>[2x]SMQDPTIFEERHLKYISQLGKGNFGSVELCRYDPLGDNTGALVAVKQLQHSGPDQQRDFQREIQILKALHSDFIVKYRGVSYGPGRQSLRLVMEYLPSGCLRDFLQRHRARLDASRLLLYSSQICKGMEYLGSRRCVHRALAARNILVESEAHVKIADFGLAKLLPLDKDYYVVREP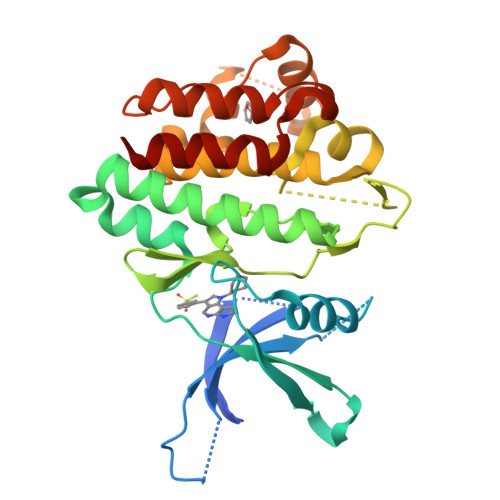GQSPIFWYAPESLSDNIFSRQSDVWSFGVVLYELFTYCDKSCSPSAEFLRMMGSERDVPALSRLLELLEEGQRLPAPPACPAEVHELMKLCWAPSPQDRPSFSALGPQLDMLWSGSR>MTQGAVKTTGKRSRAVSAKKKAILSAALDTFSQFGFHGTRLEQIAELAGVSKTNLLYYFPSKEALYIAVLRQILDIWLAPLKAFREDFAPLAAIKEYIRLKLEVSRDYPQASRLFCMEMLAGAPLLMDELTGDLKALIDEKSALIAGWVKSGKLAPIDPQHLIFMIWAST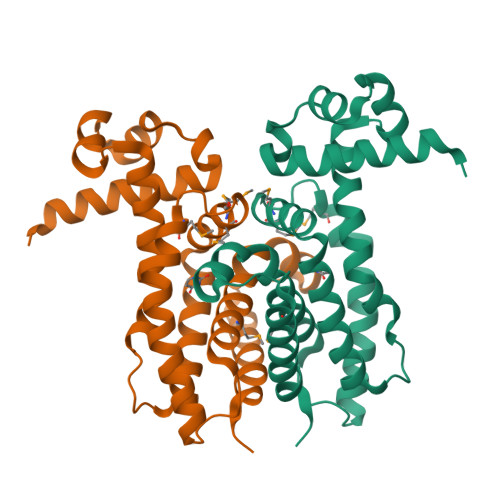QHYADFAPQVEAVTGATLRDEVFFNQTVENVQRIIIEGIRPR[4x]>GHMINYPLASSTWDDLEYKAIQSVLDSKMFTMGEYVKQYETQFAKTFGSKYAVMVSSGSTANLLMIAALFFTKKPRLKKGDEIIVPAVSWSTTYYPLQQYGLRVKFVDIDINTLNIDIESLKEAVTDSTKAILTVNLLGNPNNFDEINKIIGGRDIILLEDNCESMGATFNNKCAGTFGLMGTFSSFYNKHIATMEGGCIVTDDEEIYHILLCIRAHGWTRNLPKKNKVTGVKSDDQFEESFKFVLPGYNVRPLEMSGAIGIEQLKKLPRFISVRRKNAEYFLDKFKDHPYLDVQQETGESSWFGFSFI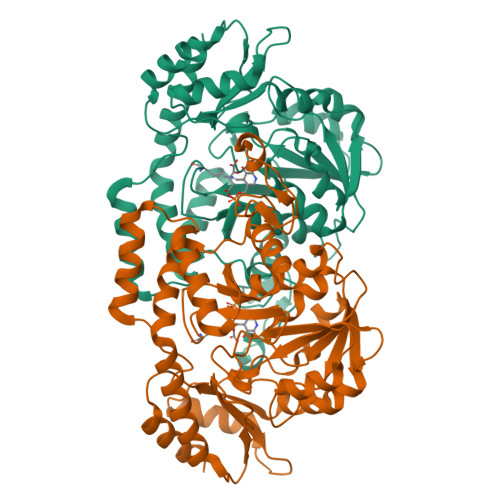IKKDSGVIRKQLVENLNSAGIECRPIVTGNFLKNTDVLKYFDYTVHNNVDNAEYLDKNGLFVGNHQIELFDEIDYLREVLK[8x]>MAGGEDRGDGEPVSVVTVRVQYLEDTDPFASANFPEPRRAPTCSLDGALPLGAQIPAVHRLLGAPLKLEDSALQVSPSGYYLDTELSLEEQREMLEGFYEEISKGRKPTLILRTQLSVRVNAILEKLYSSSGPELRRSLFSLKQIFQEDK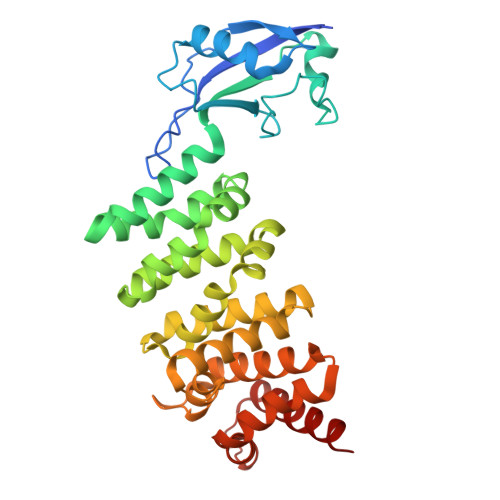DLVPEFVHSEGLSCLIRVGAAADHNYQSYILRALGQLMLFVDGMLGVVAHSDTIQWLYTLCASLSRLVVKTALKLLLVFVEYSENNAPLFIRAVNSVASTTGAPPWANLVSILEEKNGADPELLVYTVTLINKTLAALPDQDSFYDVTDALEQQGMEALVQRHLGTAGTDVDLRTQLVLYENALKLEDG[2x]> AGTALKRLMAEYKQLTLNPPEGIVAGPMNEENFFEWEALIMGPEDTCFEFGVFPAILSFPLDYPLSPPKMRFTCEMFHPNIYPDGRVCISILHAPGDDPMGYESSAERWSPVQSVEKILLSVVSMLAEPNDESGANVDASKMWRDDREQFYKIAKQIVQKSLGL;> WSADERQRMLVQ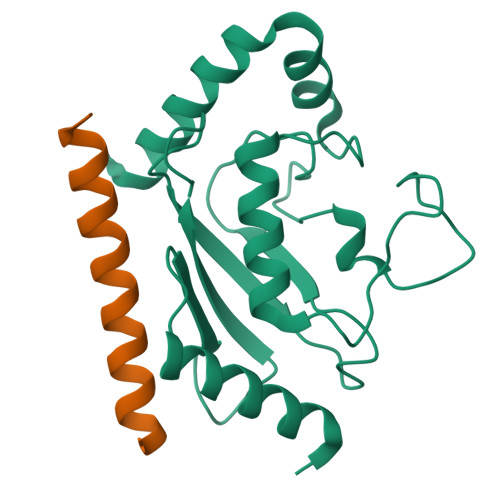RKDELLQQARKRFLNK>[3x]MVRKGEKKLAKPATTKAANPQPRRRANNRRRSNRTD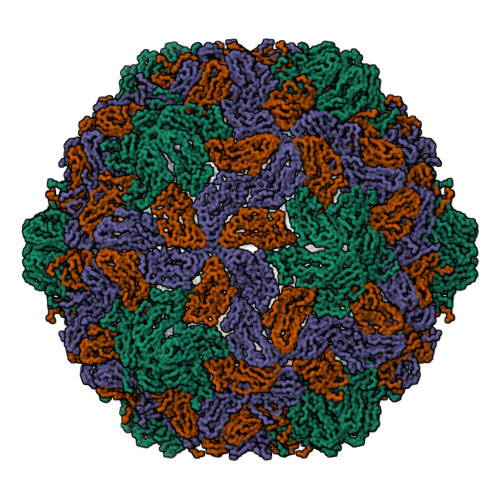APVSKASTVTGFGRGTNDVHLSGMSRISQAVLPAGTGTDGYVVVDATIVPDLLPRLGHAARIFQRYAVETLEFEIQPMCPANTGGGYVAGFLPDPTDNDHTFDALQATRGAVVAKWWESRTVRPQYTRTLLWTSSGKEQRLTSPGRLILLCVGNNTDVVNVSVLCRWSVRLSVPSLETPEETTAPIMTQGSLYNDSLSTNDFKSILLGSTPLDIAPDGAVFQLDRPLSIDYSLGTGDVDRAVYWHLKKFAGNAGTPAGWFRWGIWDNFNKTFTDGVAYYSDEQPRQILLPVGTVCTRVDSEN> HHMLHLLEQIRAYCE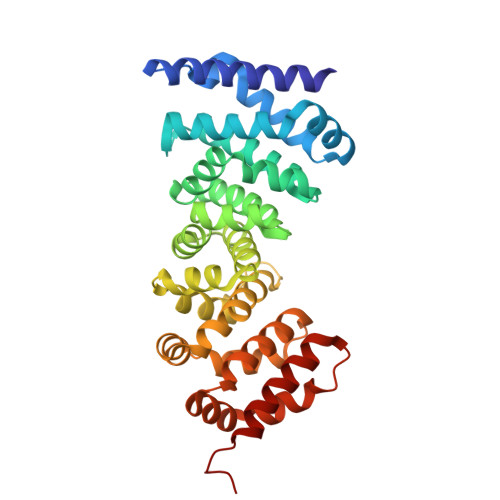TCWEWQEAHEPGMDQDKNPMPAPVEHQICPAVCVLMKLSFDEEHRHAMNELGGLQAIAELLQVDCEMYGLTNDHYSITLRRYAGMALTNLTFGDVANKATLCSMKGCMRALVAQLKSESEDLQQVIASVLRNLSWRADVNSKKTLREVGSVKALMECALEVKKESTLKSVLSALWNLSAHCTENKADICAVDGALAFLVGTLTYRSQTNTLAIIESGGGILRNVSSLIATNEDHRQILRENNCLQTLLQHLKSHSLTIVSNACGTLWNLSARNPKDQEALWDMGAVSMLKNLIHSKHKMIAMGSAAALRNLMANRPAKYK>HFQLQWPGARGAFVANDEVYFCGAHNNVTTNRTDFPLDGSGFVSIKSGHAPYTVGAIISLETDADAWEDFKNSSGGDQIAIAYRQVDN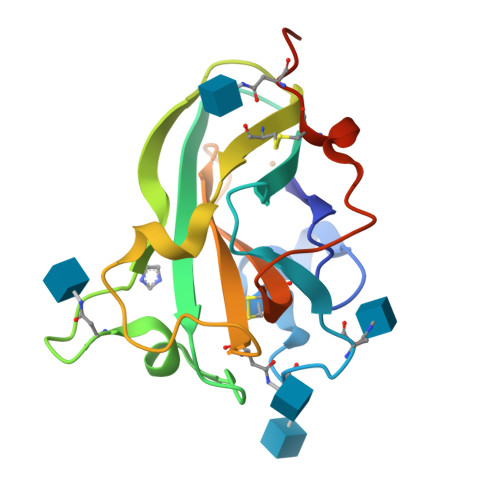SGTYCVPFNPSSLNIAGIQDGANATIQVVYTGGDGNLYQCADVTFRTTVANLNSSVCTNSTHHHHHH[2x]> MDALESLLDEVALEGLDGLCLPALWSRLETRVPPFPLPLEPCTQEFLWRALATHP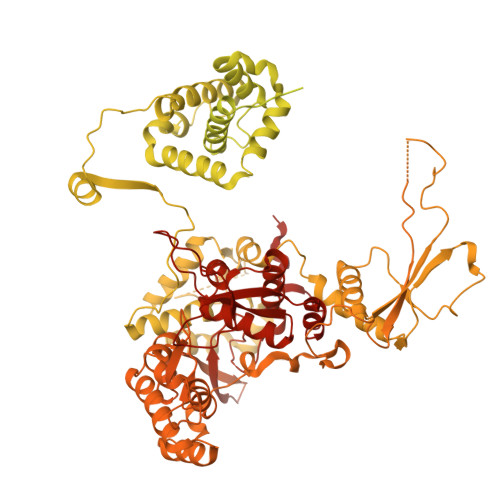GISFYEEPRERPDLQLQDRYEEIDLETGILESRRDPVALEDVYPIHMILENKDGIQGSCRYFKERKNITNDIRTKSLQPRCTMVEAFDRWGKKLIIVASQAMRYRALIGQEGDPDLKLPDFSYCILERLGRSRWQGELQRDLHTTAFKVDAGKLHYHRKILNKNGLITMQSHVIRLPTGAQQHSILLLLNRFHVDRRSKYDILMEKLSVMLSTRTNHIETLGKLREELGLCERTFKRLYQYMLNAGLAKVVSLRLQEIHPECGPCKTKKGTDVMVRCLKLLKEFKRNDHDDDEDEEVISKTVPPVDIVFERDMLTQTYDLIERRGTKGISQAEIRVAMNVGKLEARMLCRLLQRFKVVKGFMEDEGRQRTTKYISCVFAEESDLSRQYQREKARSELLTTVSLASMQEESLLPEGEDTFLSESDSEEERSSSKRRGRGSQKDTRASANLRPKTQPHHSTPTKGGWKVVNLHPLKKQPPSFPGAAEERACQSLASRDSLLDTSSVSEPNVSFVSHCADSNSGDIAVIEEVRMENPKESSSSLKTGRHSSGQDKPHETYRLLKRRNLIIEAVTNLRLIESLFTIQKMIMDQEKQEGVSTKCCKKSIVRLVRNLSEEGLLRLYRTTVIQDGIKKKVDLVVHPSMDQNDPLVRSAIEQVRFRISNSSTANRVKTSQPPVPQGEAEEDSQGKEGPSGSGDSQLSASSRSESGRMKKSDNKMGITPLRNYHPIVVPGLGRSLGFLPKMPRLRVVHMFLWYLIYGHPASNTVEKPSFISERRTIKQESGRAGVRPSSSGSAWEACSEAPSKGSQDGVTWEAEVELATETVYVDDASWMRYIPPIPVHRDFGFGWALVSDILLCLPLSIFIQIVQVSYKVDNLEEFLNDPLKKHTLIRFLPRPIRQQLLYKRRYIFSVVENLQRLCYMGLLQFGPTEKFQDKDQVFIFLKKNAVIVDTTICDPHYNLARSSRPFERRLYVLNSMQDVENYWFDLQCVCLNTPLGVVRCPRVRKNSSTDQGSDEEGSLQKEQESAMDKHNLERKCAMLEYTTGSREVVDEGLIPGDGLGAAGLDSSFYGHLKRNWIWTSYIINQAKKENTAAENGLTVRLQTFLSKRPMPLSARGNSRLNIWGEARVGSELCAGWEEQFEVDREPSLDRNRRVRGGKSQKRKRLKKDPGKKIKRKKKGEFPGEKSKRLRYHDEADQSALQRMTRLRVTWSMQEDGLLVLCRIASNVLNTKVKGPFVTWQVVRDILHATFEESLDKTSHSVGRRARYIVKNPQAYLNYKVCLAEVYQDKALVGDFMNRRGDYDDPKVCANEFKEFVEKLKEKFSSALRNSNLEIPDTLQELFARYRVLAIGDEKDQTRKEDELNSVDDIHFLVLQNLIQSTLALSDSQMKSYQSFQTFRLYREYKDHVLVKAFMECQKRSLVNRRRVNHTLGPKKNRALPFVPMSYQLSQTYYRIFTWRFPSTICTESFQFLDRMRAAGKLDQPDRFSFKDQDNNEPTNDMVAFSLDGPGGNCVAVLTLFSLGLISVDVRIPEQIIVVDSSMVENEVIKSLGKDGSLEDDEDEEDDLDEGVGGKRRSMEVKPAQASHTNYLLMRGYYSPGIVSTRNLNPNDSIVVNSCQMKFQLRCTPVPARLRPAAAPLEELTMGTSCLPDTFTKLINPQENTCSLEEFVLQLELSGYSPEDLTAALEILEAIIATGCFGIDKEELRRRFSALEKAGGGRTRTFADCIQALLEQHQVLEVGGNTARLVAMGSAWPWLLHSVRLKDREDADIQREDPQARPLEGSSSEDSPPEGQAPPSHSPRGTKRRASWASENGETDAEGTQMTPAKRPALQDSNLAPSLGPGAEDGAEAQAPSPPPALEDTAAAGAAQEDQEGVGEFSSPGQEQLSGQAQPPEGSEDPRGFTESFGAANISQAARERDCESVCFIGRPWRVVDGHLNLPVCKGMMEAMLYHIMTRPGIPESSLLRHYQGVLQPVAVLELLQGLESLGCIRKRWLRKPRPVSLFSTPVVEEVEVPSSLDESPMAFYEPTLDCTLRLGRVFPHEVNWNKWIHLGGGSGGGSGGSLEVLFQGPGSGSDYKDDDDKGDYKDDDDKGDYKDDDDK The Lon AAA+ protease (LonA) is a ubiquitous ATP-dependent proteolytic machine, which selectively degrades damaged proteins or native proteins carrying exposed motifs (degrons). LonA belongs to the AAA+ (ATPases associated with various cellular activities) superfamily and contains an N-terminal domain (NTD), a middle ATPase domain with conserved Walker motifs for ATP hydrolysis, and a C-terminal protease domain (CTD) with a serine-lysine catalytic dyad in the active site. Substrate recognition of LonA is thought to be mediated by its NTD. Collectively, our results showed that the NTD of LonA selectively interacts with protein substrates via critical hydrophobic residues of its N-lobe, demonstrating that the NTD enables LonA to perform protein quality control by selectively interacting with proteins in damaged or unfolded states.

We obtained crystals of the N-terminal fragment NN206 of MtaLonA by in situ proteolysis during crystallization. The structure was refined to 2.1 Å resolution with a free R factor of 24.9% (crystallographic R factor is 20.9%). NN206 forms a bilobal fold: (1) the N-terminal lobe, which consists of one α-helix and six β-strands, forming three β-sheets (β1/β3/β4/β5, β2/β5/β4, and β1/β6/β5); (2) the C-terminal lobe, which is exclusively α-helical, consisting of a five-helix bundle. The two lobes are jointed together by an 18-residue linker, which is similar to that of both EcLon and MacLon. Here we report the crystal structure of an N-terminal fragment of MtaLonA determined at a 2.1 Å resolution, demonstrating that it is similar to the structures of both EcLon and MacLon NTDs, but not to that of BsLon. We further applied multidimensional heteronuclear NMR experiments to assign the observed cross-peaks in 1H–15N TROSY-HSQC spectrum of NN206 (BMRB code: 50697) and the NMR-derived secondary structure of NN206, based on the Chemical Shift Index, was highly similar to its solved X-ray structures. NMR analysis indicates that thermally damaged Ig2 induces significant CSPs and broadened resonances in the NTD N-lobe, which comprises one α-helix and three β-sheets β1/β3/β4/β5, β2/β5/β4 and β1/β6/β5. The residues of MtaLonA NTD with the pronounced CSPs are part of the interaction interface located mainly at helix α1, loop L1, L2, L3, and β-sheet β2/β5/β4 (Figure 3E and Figure 3—figure supplements 3 and 4A), which consist primarily of hydrophobic residues and are decorated by a number of polar residues. By analyzing the NTD of MtaLonA interactions with damaged Ig2, the scrambled lysozyme, and Sul20 peptide, we conclude that these binding events are mediated by two hydrophobic patches, which comprise (1) L10, V14, I15, P22, V23, and M85 (termed hpI in the following); (2) M75, L77, P78, and L82 (termed hpII). In contrast, the structures of the N-terminal fragments from MtaLon, EcLon, and MacLon show that the N- and C-lobes are joined together via a short linker.

>HMRLELPVIPLRNTVILPHTTTPVDVGRAKSKRAVEEAMGADRLIFLVAQRDPEVDDPAPDDLYTWGVQAVVKQAMRLPDGTLQVMVEARARAQVTDYIPGPYLRARGEVFSEIFPIDEAVVRVLVEELKEAFEKYVANHKSLRLDRYQLEAVKGTSDPAMLADTIAYHATWTVAEKQEILELTDLEARLKKVLGLLSRDLERFELD[2x]(3E,4R,5R)-4,5-dihydroxy-3-{[(Z)-{3-hydroxy-2-methyl-5-[(phosphonooxy)methyl]pyridin-4(1H)-ylidene}methyl]imino}cyclohex-1-ene-1-carboxylic acid | C15 H19 N2 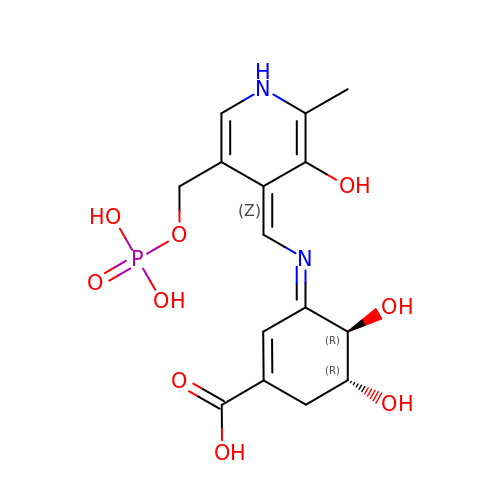O9 P | KOPNIGHVUGDBMS-FEZKIMOASA-N>[2x]PPYTVVYFPVRGRCAALRMLLADQGQSWKEEVVTVETWQEGSL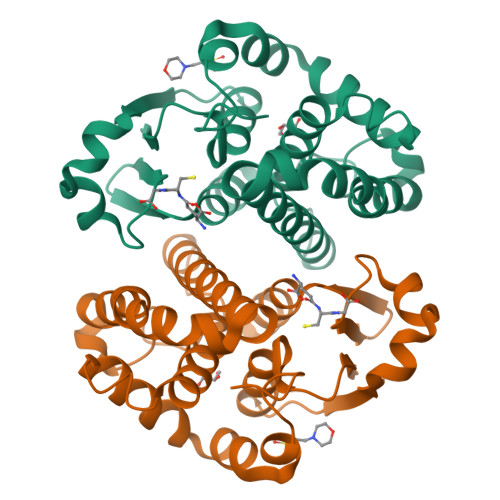KASCLYGQLPKFQDGDLTLYQSNTILRHLGRTLGLYGKDQQEAALVDMVNDGVEDLRCKYISLIYTNYEAGKDDYVKALPGQLKPFETLLSQNQGGKTFIVGDQASFADANLLDLLLIHEVLAPGCLDAFPLLSAYVGRLSARPKLKAFLASPEYVNLPINGNGKQ> NNTLWTGPKPEANCIIEYGKQNPDSKLTLILVKNGGIVNGYVTLMGASDYVNTLFKNKNVSINVELY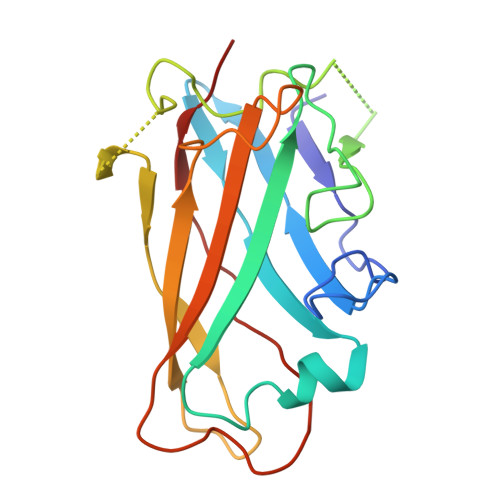FDATGHILPDSSSLKTDLELKYKQTADFSARGFMPSTTAYPFVLPNGTHNENYIFGQCYYKASDGALFPLEVTVMLNKRLPDSRTSYVMTFLWSLNAGLAPETTQATLITSPFTFSYIRED Retapamulin | C30 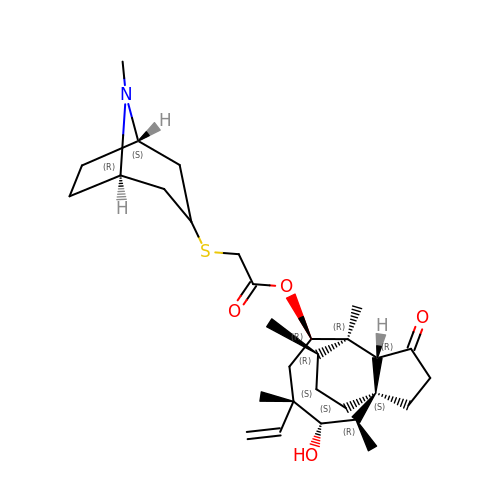H47 N O4 S | STZYTFJPGGDRJD-NHUWBDDWSA-N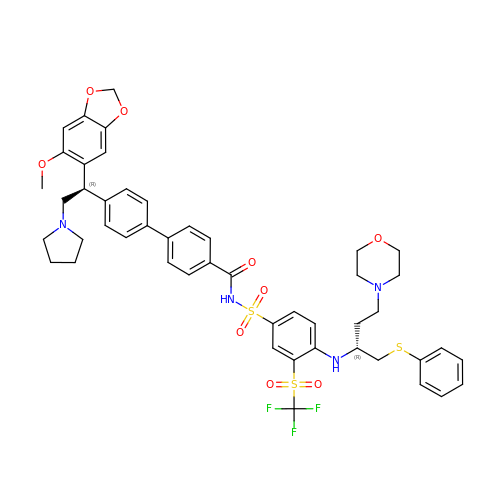4-[4-[(1~{R})-1-(6-methoxy-1,3-benzodioxol-5-yl)-2-pyrrolidin-1-yl-ethyl]phenyl]-~{N}-[4-[[(2~{R})-4-morpholin-4-yl-1-phenylsulfanyl-butan-2-yl]amino]-3-(trifluoromethylsulfonyl)phenyl]sulfonyl-benzamide | C48 H51 F3 N4 O9 S3 | VYXUKAAOZUKPPQ-GXJHCLHJSA-N> MPGLSCRFYQHKFPEVEDVVMVNVRSIAEMGAYVSLLEYNNIEGMILLSELSRRRIRSINKLIRIGRNECVVVIRVDKEKGYIDLSKRRVSPEEAIKCEDKFTKSKTVYSILRHVAEVLEYTKDEQLESLFQRTAWVFDDKYKRPGYGAYDAFKHAVSDPSILDSLDLNEDEREVLINNINRRLTPQAVKIRADIEVACYGYEGIDAVKEALRAGLNCSTENMP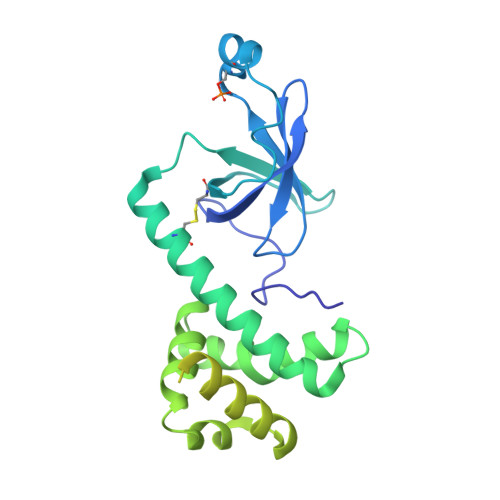IKINLIAPPRYVMTTTTLERTEGLSVLSQAMAVIKEKIEEKRGVFNVQMEPKVVTDTDETELARQMERLERENAEVDGDDDAEEMEAKAED> SEFMKIAIAGAGAMGSRFGVKLQEAGNQVTLIDNWSAHVDQINQAGLTVTTDDGVDHVYTMTAQHPEAVTDQFDLIILFTKTMQM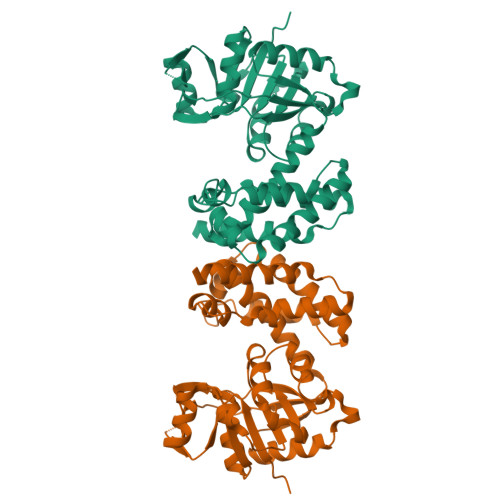DAMLQQLAPVLTNHPIVLTLANGIGNIETIERHVPKNQIVVGTTVWSSGLTGPGHITVTGTGSISLQAVVPDQFPNLADLITTLNAAGLNASAADNVLAAIWKKAGLNSVLNTYCTLFDCNIGEFGALKNWQTLTATVLDEFQAVADAAQIQFSAAAVTDLIAAQFPAAVNGNHYPSMHQDMANQRPTEIDFLNGYVAKLGQQLHVPTPANALLTQLIHSQEQLKQI The ATPase CpaF in C. crescentus is the only Tad motor reported to date that is known to be bifunctional, facilitating both pilus extension and retraction at the flagellar pole through ATP hydrolysis. CpaF oligomerization is mediated by interactions between the NTD of one chain and the CAD of an adjacent chain. From these data, we propose that CpaF uses a clockwise, rotary mechanism of catalysis to assemble a right-handed, helical Tad pilus, a process broadly applicable to other single motor systems.

In the sample without exogenous nucleotides, we resolved two distinct C2 symmetric structures, which we termed “closed” and “compact” based on the distance between symmetrically positioned residue D116 on the 3HBs, to overall resolutions of 3.4 and 3.2 Å, respectively. Thirty-six percent of the hexameric particles contributed to the reconstruction of the closed state, while 64% adopted the compact state. Nucleotide densities were not observed in the cryo-EM maps. Closed state particles were no longer observed upon the addition of nucleotides, suggesting this is strictly an apo conformation. Interestingly, two chains in the closed state adopted an ATP-bound configuration despite the absence of ATP density in the unsharpened map. Lowering the threshold of the sharpened map, however, revealed residual density in the active site, which potentially fit a diphosphate. Due to this ambiguity, coupled with the ATP-bound configuration, we designated these two chains as ATP*. The closed state of CpaF, harboring two ATP* and four Apo chains, is only observed in the absence of exogenous nucleotides, suggesting that this conformation likely does not participate in processive catalysis. In addition, the spatial position of the 3HBs in the closed state indicates that association with the platform proteins is unlikely. Thus, we hypothesize that this conformation could serve as a pre-assembly state, perhaps when the ATPase is trafficking to the poles.

>[6x]MFGKRDSSASGDPKAPPPAPAGGATIATRPQRVEPVAAPEPKAPAPKVSGPAPKPTVGLEQLRAAQGQPQTANIVREQSDYYHATKTTIFNALLNTIDLSQLAQLDLKQAGEEIRDIVAELVAIKNVSMSVAEQEHLVQDIINDVLGYGPLEPLLARDDIADIMVNGAHRVFIEVGGKVQLTNVRFRDNLQLMNICQRIVSQVGRRVDESSPICDARLPDGSRVNVIAPPLALDGPTLTIRKFKKDKLTMKNLVEFASISPEGARVLGVIGACRCNLVISGGTGSGKTTLLNTMTAFIDPTERVVTCEDAAELQLQQPHVVRLETRPPNLEGSGAVTMRDLVKNCLRMRPERIIVGEVRGPEAFDLLQAMNTGHDGSMGTLHANSPREAISRIESMITMGGYGLPSKTIKEMIVGSVDVIIQAARLRDGSRRITHITEVVGLEGDVIVTQDLFVYEITGEDEHGKVVGKHRSTGIARPRFWDRARYYGLERELAEALDAAE N-{2-[5-chloro-2-(3-chloro-5-cyanophenoxy)phenoxy]ethyl}-N-methylprop-2-enamide 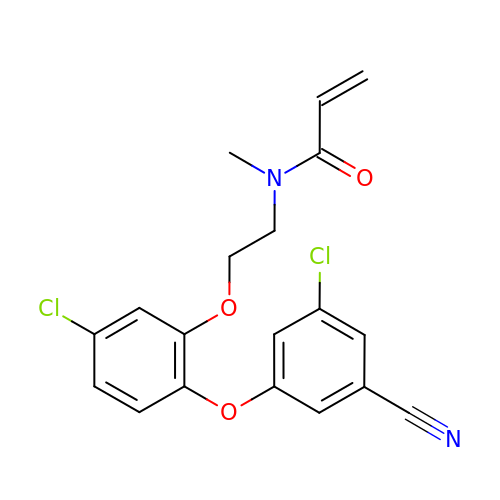| C19 H16 Cl2 N2 O3 | QOMSOHZGJXVGPQ-UHFFFAOYSA-N> MDSLSVNQILYPEVHLDSPIVTNKIVAILEYARVPHAYSLEDPTLCQNIKHRLKNGFSNQMIINNVEVGNVIKSKLRSYPAHSHIPYPNCNQDLFNIEDKESTRKIRELLKKGNSLYSKVSDKVFQCLRDTNSRLGLGSELREDIKEKVINLGVYMHSSQWFEPFLFWFTVKTEMRSVIKSQTHTCHRRRHTPVFFTGSSVELLISRDLVAIISKESQHVYYLTFELVLMYCDVIEGRLMTETAMTIDARYTELLGRVRYMWKLIDGFFPALGNPTYQIVAMLEPLSLAYLQLRDITVELRGAFLNHCFTEIHDVLDQNGFSDEGTYHELIEALDYIFITDDIHLTGEIFSFFRSFGHPRLEAVTAAENVRKYMNQPKVIVYETLMKGHAIFCGIIINGYRDRHGGSWPPLTLPLHAADTIRNAQASGDGLTHEQCVDNWKSFAGVKFGCFMPLSLDSDLTMYLKDKALAALQREWDSVYPKEFLRYDPPKGTGSRRLVDVFLNDSSFDPYDVIMYVVSGAYLHDPEFNLSYSLKEKEIKETGRLFAKMTYKMRACQVIAENLISNGIGKYFKDNGMAKDEHDLTKALHTLAVSGVPKDLKESHRGGPVLKTYSRSPVHTSTRNVRAAKGFIGFPQVIRQDQDTDHPENMEAYETVSAFITTDLKKYCLNWRYETISLFAQRLNEIYGLPSFFQWLHKRLETSVLYVSDPHCPPDLDAHIPLYKVPNDQIFIKYPMGGIEGYCQKLWTISTIPYLYLAAYESGVRIASLVQGDNQTIAVTKRVPSTWPYNLKKREAARVTRDYFVILRQRLHDIGHHLKANETIVSSHFFVYSKGIYYDGLLVSQSLKSIARCVFWSETIVDETRAACSNIATTMAKSIERGYDRYLAYSLNVLKVIQQILISLGFTINSTMTRDVVIPLLTNNDLLIRMALLPAPIGGMNYLNMSRLFVRNIGDPVTSSIADLKRMILASLMPEETLHQVMTQQPGDSSFLDWASDPYSANLVCVQSITRLLKNITARFVLIHSPNPMLKGLFHDDSKEEDEGLAAFLMDRHIIVPRAAHEILDHSVTGARESIAGMLDTTKGLIRASMRKGGLTSRVITRLSNYDYEQFRAGMVLLTGRKRNVLIDKESCSVQLARALRSHMWARLARGRPIYGLEVPDVLESMRGHLIRRHETCVICECGSVNYGWFFVPSGCQLDDIDKETSSLRVPYIGSTTDERTDMKLAFVRAPSRSLRSAVRIATVYSWAYGDDDSSWNEAWLLARQRANVSLEELRVITPISTSTNLAHRLRDRSTQVKYSGTSLVRVARYTTISNDNLSFVISDKKVDTNFIYQQGMLLGLGVLETLFRLEKDTGSSNTVLHLHVETDCCVIPMIDHPRIPSSRKLELRAELCTNPLIYDNAPLIDRDATRLYTQSHRRHLVEFVTWSTPQLYHILAKSTALSMIDLVTKFEKDHMNEISALIGDDDINSFITEFLLIEPRLFTIYLGQCAAINWAFDVHYHRPSGKYQMGELLSSFLSRMSKGVFKVLVNALSHPKIYKKFWHCGIIEPIHGPSLDAQNLHTTVCNMVYTCYMTYLDLLLNEELEEFTFLLCESDEDVVPDRFDNIQAKHLCVLADLYCQPGTCPPIQGLRPVEKCAVLTDHIKAEAMLSPAGSSWNINPIIVDHYSCSLTYLRRGSIKQIRLRVDPGFIFDALAEVNVSQPKIGSNNISNMSIKAFRPPHDDVAKLLKDINTSKHNLPISGGNLANYEIHAFRRIGLNSSACYKAVEISTLIRRCLEPGEDGLFLGEGSGSMLITYKEILKLSKCFYNSGVSANSRSGQRELAPYPSEVGLVEHRMGVGNIVKVLFNGRPEVTWVGSVDCFNFIVSNIPTSSVGFIHSDIETLPDKDTIEKLEELAAILSMALLLGKIGSILVIKLMPFSGDFVQGFISYVGSHYREVNLVYPRYSNFISTESYLVMTDLKANRLMNPEKIKQQIIESSVRTSPGLIGHILSIKQLSCIQAIVGDAVSRGDINPTLKKLTPIEQV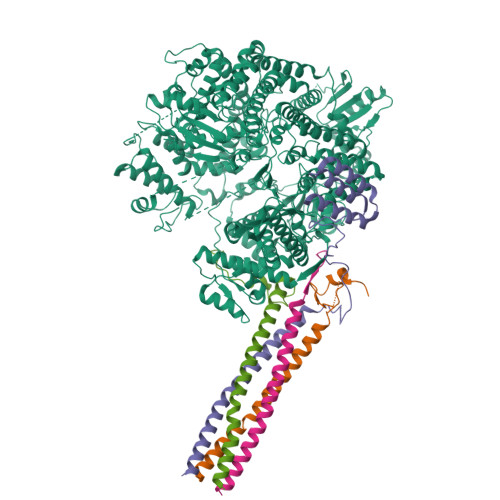LINCGLAINGPKLCKELIHHDVASGQDGLLNSILILYRELARFKDNQRSQQGMFHAYPVLVSSRQRELISRITRKFWGHILLYSGNRKLINKFIQNLKSGYLILDLHQNIFVKNLSKSEKQIIMTGGLKREWVFKVTVKETKEWYKLVGYSALIKD;>[4x]MAEEQARHVKNGLECIRALKAEPIGSLAIEEAMAAWSEISDNPGQERATCREEKAGSSGLSKPCLSAIGSTEGGAPRIRGQGPGESDDDAETLGIPPRNLQASSTGLQCHYVYDHSGEAVKGIQDADSIMVQSGLDGDSTLSGGDNESENSDVDIGEPDTEGYAITDRGSAPISMGFRASDVETAEGGEIHELLRLQSRGNNFPKLGKTLNVPPPPDPGRASTSGTPIKKGTDARLASFGTEIASSLTGGATQCARKSPSEPSGPGAPAGNVPECVSNAALIQEWTPESGTTISPRSQNNEEGGDHYDDELFSDVQDIKTALAKIHEDNQKIISKLESLLLLKGEVESIKKQINRQNISISTLEGHLSSIMIAIPGLGKDPNDPTADVEINPDLKPIIGRDSGRALAEVLKKPVASRQLQGMTNGRTSSRGQLLKEFQLKPIGKKMSSAVGFVPDTGPASRSVIRSIIKSSRLEEDRKRYLMTLLDDIKGANDLAKFHQMLMKIIMKSG> GAMGSKSQQPLQNLSHSPSYTENKPDKKKKYMINDAKTIQLVGPLISSPDNLGFQKRSHKARELPRFLINQEPQLEKRAFVQDPWDKANQEKMISLEESIDDLNELYETLKKMRNTERSIMEEKGLVDKADSAKDLYDAIVFQGTCLDMCPTFERSRRNVEYTVYSYEKNQPNDKKASRTKALKVFARPAAAAAPPLPSDVRPPHILVKTLDYIVDNLLTTLPESEGFLWDRMRSIRQDFTYQNYSGPEAVDCNERIVRIHLLILHIMVKSNVEFSLQQELEQLHKSLITLSEIYDDVRSSGGTCPNEAEFRAYALLSKIRDPQYDENIQRLPKHIFQDKLVQMALCFRRVISNSAYTERGFVKTENCLNFYARFFQLMQSPSLPLLMGFFLQMHLTDIRFYALRALSHTLNKKHKPIPFIYLENMLLFNNRQEIIEFCNYYSIEIINGDAADLKTLQHYSHKLSETQPLKKTYLTCLERRLQKTTYKGLINGGEDN;> MDMANQLLDELAHGNFSHLTLNLSQNGREIAIL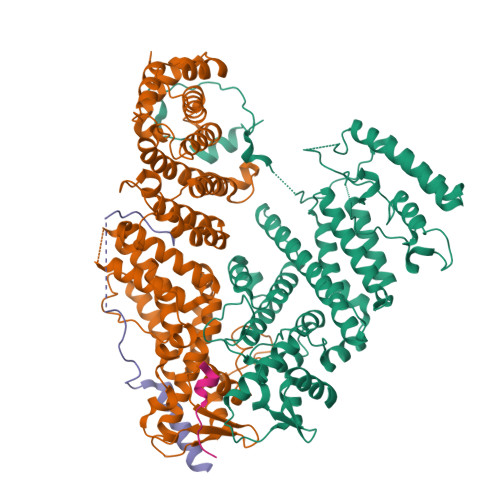QKQLTGFDDKQLETFVEQHPAMPNDTRFKIMCTSFLNYARDVDPWSAWSSSDLIFEFYQCLINCLINDNAPHIEMLIPVATRETEFIINLAGKLDSFHLQLHTRSHQFLSHISSILSRLFNSIKPPRGNASSTNIPGKQRILLYLVNKLNNIYFRIESPQLCSNIFKNFQPKSMLAHFNEYQLDQQIEYRYLLGRYYLLNSQVHNAFVQFNEAFQSLLNLPLTNQAITRNGTRILNYMIPTGLILGKMVKWGPLRPFLSQETIDNWSVLYKHVRYGNIQGVSLWLRQNERHLCARQLLIVLLEKLPMVTYRNLIKTVIKSWTTEWGQNKLPYSLIERVLQLSIGPTFEDPGAQEITIYNGIHSPKNVENVLVTLINLGLLRANCFPQLQLCVVKKTTMIQEIVPPVNERITKMFPAHSHVLW;> MSTDVAAAQAQSKIDLTKKKNEEINKKSLEEDDEFEDFPIDTWANGETIKSNAVTQTNIWEENWDDVEVDDDFTNELKAELDRYKRENQ;> MSHEGEEDLLEYSDNEQEIQIDASKAAEAGETGAATSATEGDNNNNTAAGDKKGS>[4x]MTSVQLETPHSGKYEQPTGLFINNEFVKGQEGKTFDVINPSDESVITQVHEATEKDVDIAVAAARKAFEGSWRQETPENRGKLLNNLANLFEKNIDLLAAVESLDNGKAISMAKGDISMCVGCLRYYGGWADKITGKVIDTTPDTFNYVKKEPIGVCGQIIPWNFPLLMWAWKIGPAIACGNTVVLKTAEQTPLGGLVAASLVKEAGFPPGVINVISGFGKVAGAALSSHMDVDKVAFTGSTVVGRTILKAAASSNLKKVTLELGGKSPNIVFEDADIDNAISWVNFGIFFNHGQCCCAGSRVYVQESIYDKFVQKFKERAQKNVVGDPFAADTFQGPQVSKVQFDRIMEYIQAGKDAGATVETGGKRKGDKGYFIEPTIFSNVTEDMKIVKEEIFGPVCSIAKFKTKEDAIKLGNASTYGLAAAVHTKNLNTAIEVSNALKAGTVWVNTYNTLHHQMPFGGYKESGIGRELGEDALANYTQTKTVSIRLGDALFG

Many protein families have numerous members listed in databases as allergens; however, some allergen database entries, herein called “orphan allergens”, are members of large families of which all other members are not allergens. Three orphan allergens [Cladosporium herbarum aldehyde dehydrogenase (ChALDH), Alternaria alternata ALDH (AaALDH), and C. herbarum mannitol dehydrogenase (ChMDH)] were recombinantly produced and purified for structure characterization and for clinical skin prick testing (SPT) in mold allergic participants. Diffraction quality crystals of ChALDH and ChMDH were obtained, and their X-ray crystal structures were determined by molecular replacement. Examination of the X-ray crystal structures of ChALDH and ChMDH and a homology structure model of AaALDH did not identify any discernable epitopes that distinguish these putative orphan allergens from their non-allergenic protein relatives.

ChALDH and AaALDH are both tetrameric proteins with monomers of Mr ~ 54 kDa and are members of the ALDH enzyme family, which catalyze the oxidation of aldehydes to carboxylic acids and are found across multiple prokaryote and eukaryote species. The 3.18 Å resolution structure of ChALDH revealed a tetrameric structure, which corresponded with the size-exclusion chromatography analysis of the purified protein. Each monomer unit of ChALDH retains the canonical ALDH domain organization of catalytic, NAD(P)(H) binding, and oligomerization domains. The secondary structure domains of ChALDH have high similarity to those of other ALDH, including the catalytic residues in the active site and the nucleotide cofactor binding site. Although no ligand was bound in the ChALDH structure, amino acid residues formed interactions where a computationally docked NADP+ molecule is in the active site. The active site of ChALDH would form extensive van der Waals interactions with the adenine ring and nicotinamide ring of the cofactor, which is proximate to the catalytic cysteine (Cys296). Hydrogen bonds between the adenine-ribose ring and Ile161 and Lys187, as well as Trp163 and Ser241 interacting with the cofactor phosphate groups. The overall fold of the ChALDH monomer shares structural similarities with other ALDH family members from both prokaryotes and eukaryotes, which range in sequence identity from 32 to 57% and with root mean square deviations (r.m.s.d.) of 0.8–1.6 Å for 460–469 Cα-atoms. Not unexpectedly, structural alignment of ChALDH with the ALDHs from maize (51% identity), spinach (43% identity), and tomato (51% identity) shows the conservation of the overall three-dimensional fold of these enzymes. In addition, there is little variation in either the surface electrostatics or surface hydrophobicity between ChALDH, AaALDH, and the representative ALDHs from maize, spinach, and tomato.MpPA14 (Marinomonas primoryensis PA14 domain) lectin is a domain of a 1.5-MDa adhesin responsible for a symbiotic bacterium-diatom interaction in Antarctica. Bioinformatic analyses indicated the presence of an ∼20-kDa domain near the C terminus of MpIBP that is a member of the PA14 family, which is a carbohydrate-binding lectin module widely distributed across several kingdoms of life. PA14 domains share a β-sandwich fold and the presence of two consecutive aspartate residues in a cis peptide linkage (DcisD). The DcisD motif coordinates a Ca2+ ion that is directly involved in binding polar vicinal hydroxyl groups of various carbohydrates.

We further analyzed the crystal structures of MpPA14 in complex with three pentoses, l-arabinose, ribose, and 2-deoxy-ribose, as well as inositol, which has an unusual 6-carbon saccharide ring without an endocyclic oxygen. These four carbohydrates bound MpPA14 more weakly than glucose and mannose. Crystal structures showed that MpPA14 selects the pyranose form of pentoses for binding. As pentoses have a higher percentage of furanose present in the conformational equilibria than do hexoses, selectivity for the more thermodynamically stable pyranoses might contribute to the weaker affinity of pentoses toward the lectin. For instance, despite l-arabinose existing in solution predominantly in the pyranose form at 25°C (57% α-arabinopyranose versus 30.5% β-arabinopyranose), only the α-anomer complexes MpPA14 via its 1,2-diol. For instance, while arabinan is a polymer of arabinose, a sugar that MpPA14 binds, X-ray crystallography showed that MpPA14 is selective in only forming a complex with α-l-arabinopyranose. This conformer is not present in the arabinan polymer composed of 1,5-linked α-l-arabino-furanoses, which are then not free to transition to the pyranose form.

> QDDSTPDSLFAGLVGEYYGTNSQLNNISDFRALVDSKEADATFEAANISYGRGSSDVAKGTHLQEFLGSDASTLSTDPGDNTDGGIYLQGYVYLEAGTYNFKVTADDGYEITINGNPVATVDNNQSVYTVTHASFTISESGYQAIDMIWWDQGGDYVFQPTLSADGGSTYFVLDSAILSSTGETPYTTAQ>MSLSTRIAPHLPYLRRFARSVTGSQSSGDAYVSAMLEALIADISIFPRASSDRIGTYWLFCHLFDQTTPNIPEPLPQFGLEQKTSAKLSYLTPRARQAFLLIAVEGFNEQEASEIMNLDARDFRKLLNQASIDISQQIATQVMIIEDEPLIAMDIEQMVESLGHQVVGIARTRKEAVVMYHQKKPRLILADIQLADNSSGIDAVNDILQNDRIPVIFITAFPERLLTGERPEPTFLVTKPFNPDMVKALISQALFFKENASKAALEAGWSHPQFEK[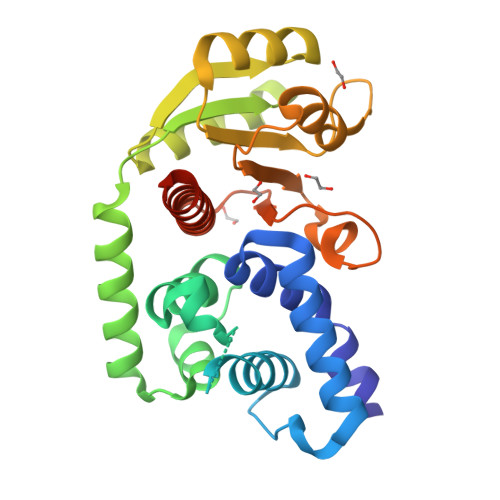2x]> MPISPIETVPVKLKPGMDGPKVKQWPLTEEKIKALVEICTEMEKEGKISKIGPENPYNTPVFAIKKKDSTKWRKLVDFRELNKRTQDFWEVQLGIPHPAGLKKKKSVTVLDVGDAYFSVPLDEDFRKYTAFTIPSINNETPGIRYQYNVLPQGWKGSPAIFQSSMTKILEPFRKQNPDIVIYQYMDDLYVGSDLEIGQHRTKIEELRQHLLRWGLTTPDKKHQKEPPFLWMGYELHPDKWTVQPIVLPEKDSWTVNDICKLVGKLNWASQIYPGIKVRQLSKLLRGTKALTEVIPLTEEAELELAENREILKEPVHGVYYDPSKDLIAEIQKQGQGQWTYQIYQEPFKNLKTGKYARMRGAHTNDVKQLTEAVQKITTESIVIWGKTPKFKLPIQKETWETWWTEYWQATWIPEWEFVNTPPLVKLWYQLEKEP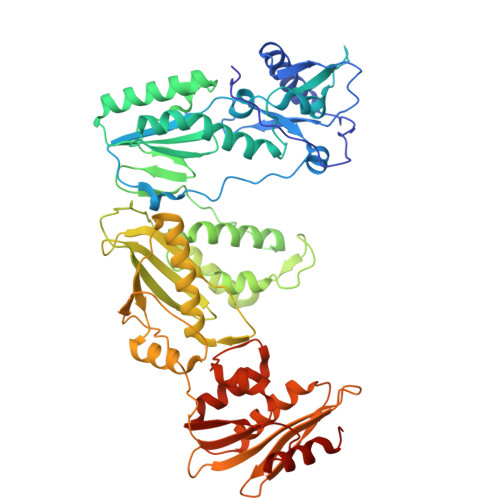IVGAETFYVDGAANRETKLGKAGYVTNRGRQKVVTLTDTTNQKTELQAIYLALQDSGLEVNIVTDSQYALGIIQAQPDQSESELVNQIIEQLIKKEKVYLAWVPAHKGIGGNEQVDKLVSAGIRKVL>[2x]PSVYDAAAQLTADVKKDLRDSWKVIGSDKKGNGVALMTTLFADNQETIGYFKRLGDVSQGMANDKLRGHSITLMYALQNFIDQLDNPDDLVCVVEKF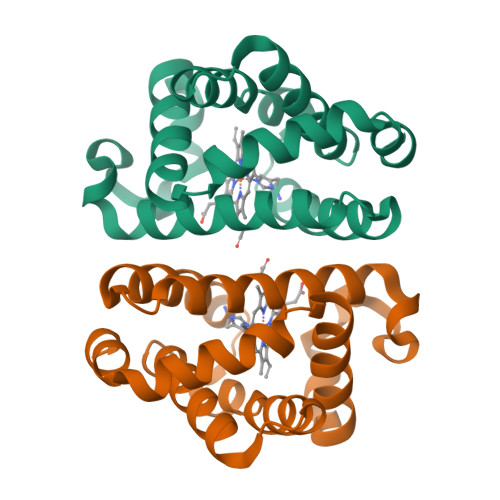AVNHITKKISAAEFGKINGPIKKVLASKNFGDKYANAWAKLVAVVQAAL>[2x]GPGSMLSEQQYRIEHDTMGEVRVPAEALW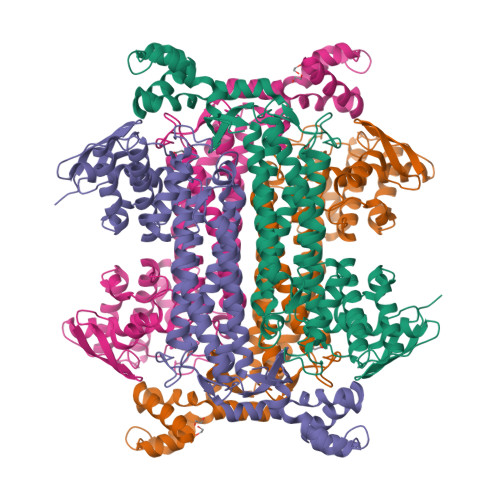RAQTQRAVENFPISGRGLERTQIRALGLLKGACAQVNKDLGLLAAEKADAIIAAAQEIADGKHDDQFPIDVFQTGSGTSSNMNANEVIASIAAQATPPVVVHPNDDVNMSQSSNDTFPTATHLAATEAAVRDLIPALEYLQQALATKAKAWKTVVKSGRTHLMDAVPVTLGQEFGGYARQIEAGIERVKATLPRLGELPIGGTAVGTGLNAPDGFGAKVVEVLKQSTGLSELKTASDSFEAQAARDGLVEGSGALKTIAASLTKIANDIRWMGSGPLTGLGEIQLPDLQPGSSIMPGKVNPVLPEAVTQVAAQVIGNDAAITVGGLSGAFELNVYIPVMARNLLESFTLLANVSRLFVDKCVDGLVANEDHLRTLAESSPSIVTPLNSAIGYEEAAAVAKEALKERKTIRQTVIDRGLIGDKLSIEELDKRLDVLAMAKVKD>MHHHHHHSTPSIVIASAARTAVGSFNGAFANTPAHELGATVISAVLERAGVAAGEVNEVILGQVLPAGEGQNPARQAAMKAGVPQEATAWGMNQLCGSGLRAVALGMQQIATGDASIIVAGGMESMSMAPHCAHLRGGVKMGDFKMIDTMIKDGLTDAFYGYHMGTTAENVAKQWQLSRDEQDAFAVASYNKAEAAQKDGRFKDEIVPFIVKGRKGDITVDADEEIRGATLDKMAKLRPAFDKEGTVTAGNASGLNDGAAAALLMSEAEASRRGIQPLGRIVSWATVGVDPKVMGTGPIPASRKALERAGWKIGDLDLVEANEAFAAQACAVNKDLGWDPSIVNVNGGAIAIGHPIGASGARI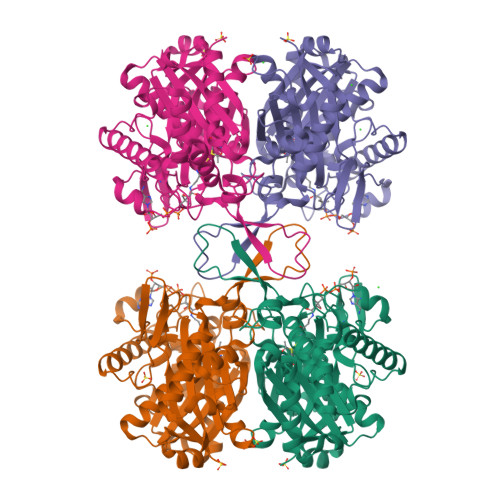LNTLLFEMKRRGARKGLATLCIGGGMGVAMCIESL[4x]>[4x]MSEQKQDVAATEEQQPVLQIQRIYVKDVSFEAPNLPHIFQQEWKPKLGFDLSTETTQVGDDLYEVVLNISVETTLEDSGDVAFICEVKQAGVFTISGLEDVQMAHCLTSQCPNML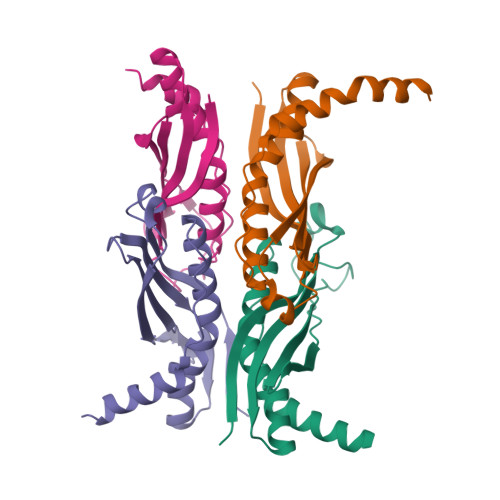FPYARELVSNLVNRGTFPALNLSPVNFDALFVEYMNRQQAENAEEKSEEEQTKH> EEFDPELAREVEDLRQRDQVTGLLNRPTFMVALEQAVAQAGRSEGQSGFLLIEPDHYARILPEFGLDSADALIAALAAHVASVLDDSVLAARFGEHSFALLLNGNYARTHALAETVRNAFAQHVFSVGTRSATVTVSIGGVQIGEKIASIGQVLNRGTEAVRTTAELGGNAVSIYDPAAADRAEEERIERWVEQLREALVGDGFLLHYQPVLNLQGEPLELYQAFLRLERNGEMMSPNAFMAIAEEHDLVTEIDRWVVARAIRQLGERQRAGHKTHLLVRIGPNSFSDPQMIDTIREQLAVYGVPGERLWLQTPESKVFTHLRNAQQFLAAVSAMDCKVGLEQFGSGLDSFQLLAHFHPAFLKLDRGITGDIASARDSQEKIREITSRAQPAGILTMAEFVADAQSMSSFFSAGVDYVQGDFVAPTGPLMNYEFG;> MSAMNARQGILSLALKDKPALYSAYMPFVKGGGIFVPTPKRYMLGDEVFLLLTLPDSSERLPVAGKVIWTTPAGAQGNRAAGIGVQFPDGPEGEAVRNKIETLLAG

Type IV pili (T4P) are thin and flexible filaments found on the surface of a wide range of Gram-negative bacteria that undergo cycles of extension and retraction and participate in a variety of important functions related to lifestyle, defense and pathogenesis. T4P filaments are produced by the polymerization of pilin subunits in a process that depends on PilB, a hexameric ATPase associated with the bacterial inner membrane, while pilus retraction is powered by another hexameric ATPase, PilT. In Xanthomonas citri, two cytosolic proteins, PilZ and the c-di-GMP receptor FimX, are involved in the regulation of T4P biogenesis through interactions with PilB.

We also crystallized the complex between PilZΔ107–117 and a larger FimX fragment encompassing its GGDEF and EAL domains (FimXGGDEF-EAL, residues 255–689) in the presence of c-di-GMP. The PilZΔ107-117-FimXGGDEF-EAL complex crystallized in space group P42212 with one copy of each protein in the asymmetric unit (see S1 Table for data collection statistics). Very clear electron density for PilZΔ107–117 and the FimX EAL domain (beginning at residue 436) with bound c-di-GMP in the syn/anti conformation were observed. However, no density for the FimX GGDEF domain could be detected, a phenomenon similar to that observed for the crystal structure of the FimXGGDEF-EAL fragment from P. aeruginosa that is only 30% identical to X. citri FimXGGDEF-EAL. The PilZΔ107-117-FimXGGDEF-EAL crystal presents the same two principal modes of crystal lattice contacts between PilZ and the FimX EAL domain observed in the previously published PilZ-FimXEAL crystal structures from X. citri and X. campestris, in spite of the different fragments used and different space groups. We name these two modes of contact interfaces 1 and 2. The most significant difference among the three structures has to do with the orientation of the first helix in FimXEAL domains: in the X. citri PilZ-FimXEAL and PilZΔ107-117-FimXGGDEF-EAL complexes (residues 429–454 and 436–454, respectively), the helix is oriented so as to contribute significantly to the interaction with PilZ in interface 1 (362 or 308 Å2 and 234 Å2 of buried surface, respectively) while this helix is rotated approximately 140o, pointing away from PilZ in the X. campestris PilZ-FimXEAL structure. While interface 1 involves a β-sheet extension and tenuous contacts between PilZ and the c-di-GMP ligand bound to FimX, interface 2 is dominated by hydrophobic interactions. We note that the binary complexes employing wild-type and D46A/E47A PilZ seem to be stabilized by the addition of c-di-GMP. Together, these observations raise the possibility that interface 2 between PilZ and FimX EAL domains may be physiologically relevant.> MSNNLFGTGSSTSSSLFGSTPSAGGLFGGGSSTTPATGGGGLFGGASTTPATGGGLFGGASTTPATGGGLFGGASTTPATGGGGLFGGSSTTAPATGGGGLFGGSTTTAPATTGGLFGGSSTTAPSTTTGGLFGGSSTTTPSITTTGGLFGGASTTAPSTTTGGLFGATTPATTATTTTGGLFGGSTTTPSLTSGGGLFGATTPAATTTTTSSAIPSLTSGGGLFGGSTTTPSLTSGGLFGATTPAATTTTSTTTPSLTSGGLFGATTPSTTGGLFGASTTTTTTPSTTSTTTPSTTTGGLFGATTPATTTTSGGLFGASTTTPSTTGGLFGVSTTTPSTTSATTPTTTTTGGLFGAATTSATTPSTTTTTTTTTPTTGLFGSSTTPSTTTSGGLFGSSTTPSTTTTTTTATTPTTGGLFGSSTTPSTTTTSGGLFGSSATPSTTSSGGLFGATTTSATTTTTTPTTTSGGLFGTSSTTTTTTTPAAVAATSSNPLTTSMLGGSSTTPNPVSASLNNSDPIGINESKLLEQLLNEWVSEIENQ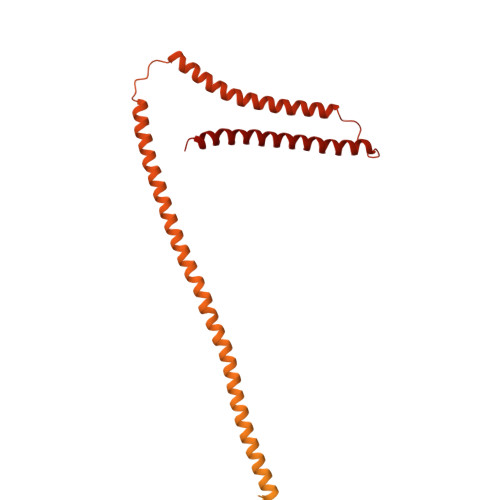TKNFYDQAKTIFVWDQRIMDNSQKLGKLMDVVVKLNSQQNALNQCIDVVRDQQALLERSLNALDSKIKSSPKDNETTADLERERIYSLATKIDDDIIKVENKLLGVVNKINQNQVKDDNPKDLNQKVSKILNDHLNTLQWIDKSTNILQESLKVIESTSLPETSRR O-SULFO-L-SERINE 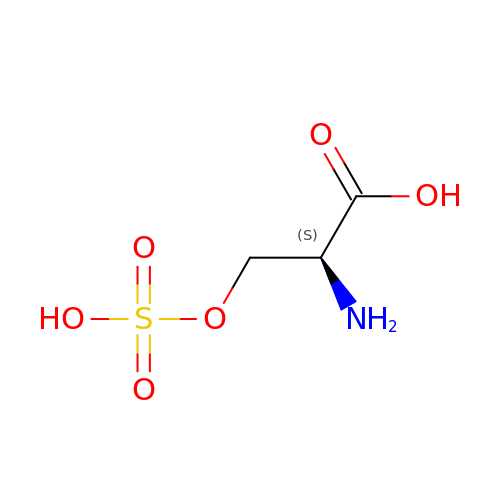| C3 H7 N O6 S | LFZGUGJDVUUGLK-REOHCLBHSA-N> SLSCDRNGICKGSSGSLNSIPSGLTEAVKSLDLSNNRITYISNSDLQRCVNLQALVLTSNGINTIEEDSFSSLGSLEHLDLSYNYLSNLSSSWFKPLSSLTFLNLLGNPYKTLGETSLFSHLTKLQILRVGNMDTFTKIQRKDFAGLTFLEELEIDASDLQSYEPKSLKSIQNVSHLILHMKQHILLLEIFVDVTSSVECLELRDTDLDTFHFSELSTGETNSLIKKFTFRNVKITDESLFQVMKLLNQISGLLELEFDDCTLNGVGNFRASDNDRVIDPGKVETLTIRRLHIPRFYLFYDLSTLYSLTERVKRITVENSKVFLVPCLLSQHLKSLEYLDLSENLMVEEYLKNSACEDAWPSLQTLILRQNHLASLEKTGETLLTLKNLTNIDISKNSFHSMPETCQWPEKMKYLNLSSTRIHSVTGCIPKTLEILDVSNNNLNLFSLNLPQLKELYISRNKLMTLPDASLLPMLLVLKISRNQLKSVPDGIFDRLTSLQKIWLHTNPWDCSCPRIDYLSRWLNKNSQKEQGSAKCSGSGKPVRSIICP;> SEFLVDRSKNGLIHVPKDLSQKTTILNISQNYISELWTSDILSLSKLRILIISHNRIQYLDISVFKFNQELEYLDLSHNKLVKISCHPTVNLKHLDLSFNAFDALPICKEFGNMSQLKFLGLSTTHLEKSSVLPIAHLNISKVLLVLGETYGEKEDPEGLQDFNTESLHIVFPTNKEFHFILDVSVKTVANLELSNIKCVLEDNKCSYFLSILAKLQTNPKLSNLTLNNIETTWNSFIRILQLVWHTTVWYFSISNVKLQGQLDFRDFDYSGTSLKALSIHQVVSDVFGFPQSYIYEIFSNMNIKNFTVSGTRMVHMLCPSKISPFLHLDFSNNLLTDTVFENCGHLTELETLILQMNQLKELSKIAEMTTQMKSLQQLDISQNSVSYDEKKGDCSWTKSLLSLNMSSNILTDTIFRCLPPRIKVLDLHSNKIKSIPKQVVKLEALQELNVASNQLKSVPDGIFDRLT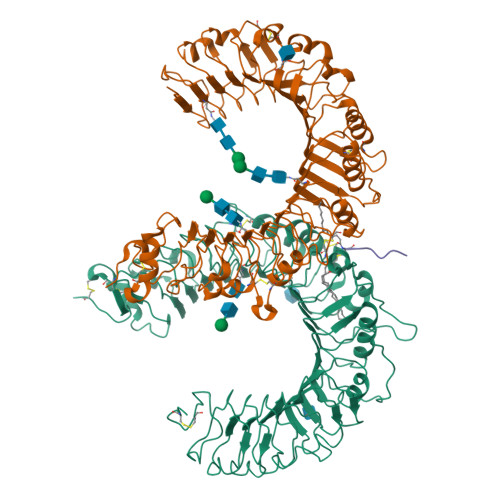SLQKIWLHTNPWDCSCPRIDYLSRWLNKNSQKEQGSAKCSGSGKPVRSIICP;> CSKKKK NbUGT72AY1 is a promiscuous transferase that glycosylates bioactive hydroxycoumarins such as scopoletin and umbelliferone, as well as monolignols involved in lignin formation and various other small molecules. Five distinct GT protein folds have been identified that are capable of GT activity (termed GT-A to GT-E). NbUGT72AY1 adopts a GT-B fold comprised of two distinct N-terminal and C-terminal Rossmann-like domains (shown in cyan and brown in Fig. 2, respectively) of seven and six parallel β-sheets, respectively linked to α-helices, connected by a linker region and an interdomain cleft. The catalytic mechanism of inverting UGT such as NbUGT72AY1 is a direct displacement bimolecular nucleophilic substitution (SN2)-like reaction enabled by an enzymatic base catalyst.

Moreover, NbUGT72AY1 crystallized in the presence of scopoletin (III), UDP (IV), and a mixture of scopoletin and the non-transferable donor UDP2FG (V). Complex V and IV represent the SI and product-inhibited enzyme complexes, respectively, as they were obtained in the presence of an excess of substrate (scopoletin) and product (UDP), respectively. Asn372, Ser373, Glu376, Arg249, Ala351, and Trp350 frame their donor binding sites and in both structures, the indole ring of Trp350 points in the direction towards the uracil structure of UDP2FG and UDP, resulting in a π-stacking interaction. In all UDP/UDP2FG-bound structures (IV, V, VI, and VII), the indole ring system of Trp350 forms a π interaction with the uracil ring. In all structures that have scopoletin bound (III, V, VI, VIII, and IX), H2 has 2-3 turns while conformers associated with UDP (IV) and UDP2FG (VII) have 4 turns. The product inhibited protein structure IV and SI complex V show closed active sites with distinct electron densities for the residues from 310-326 in IV and V, while catalytically active VI and VII lack electron densities for this region due to the high dynamics and the loop may remain open. The non-productive complexes IV and V are compact, fully resolved, and display a closed active site. Phe53, an amino acid of helix H2, interacts via π-cation binding with Arg214 of the UDPG-binding pocket and approaches Trp350 4.1 Å in SI complex V and 4.0 Å in the product-inhibited structure IV, while the distance is larger in all other structures. Aside from the closed active site, the amino acids in the nonfunctional structures move closer together, resulting in a more compact complex and a higher number of non-covalent interactions. The lowest number of interactions (total edges) was calculated for the protein in the presence of β-carotene (II), while the highest number of bonds was obtained after addition of UDP (IV_A and IV_B), which is consistent with the assumption that the carotenoid promotes protein dynamics, while in the product-inhibited complex the mobility of the protein is hindered.

>[2x]MDSSQLHVAIVSSPGMGHLIPVLVLGNRLATHHNIKITILAITTTSSSAETEFLKKTTLTNEEKTIEIIPVPSVDISHLINSSTKIFTQLRLLVREALPKIHSTIASMTHRPDALIVDIFCTQILPIAEEFNISKYTYHPTTAWTLALAIYCQVFDKEIEGEYVELKEPLKIPGCKALRPDDVVDPLLDRSDQQYEEYVKLGKEYTDFDGILINTWEDLEPETINALRYNEKLRLLLKVPVFPIGPLRRKVETTLNDEVIQWLDKQNNESVLFVSFGSGGTLSTKQMTELAWGLELSQQKFVWVVRPPSDGDADSAYLNSAGKDTRDMSEYLPEGFLTRTKDMGLVVPMWANQVEILSHSSVGGFLTHCGWNSTVESLTNGVPMIAWPLHAEQKMNAAMLTEELGVAIRPAVLPTKKLVKREEIQGMVRILMQTKEGKRIKEKAKKLKKSAENALSDGGSSYNSICELVKDIRSREL(3Z)-N-[(1R)-1-(4-fluorophenyl)ethyl]-3-({4-[(furan-2-carbonyl)amino]-3,5-dimethyl-1H-pyrrol-2-yl}methylidene)-2-oxo-3,7-dihydro-2H-indole-5-carboxamide 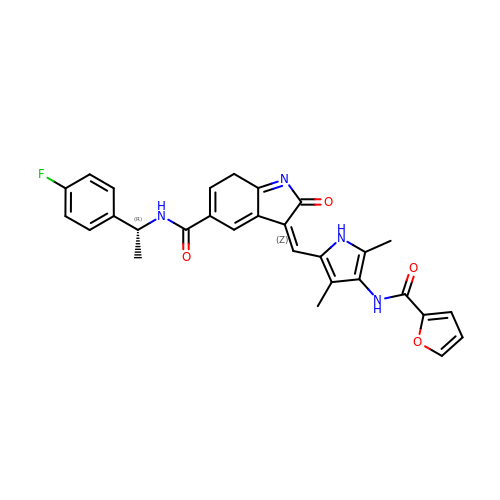| C29 H25 F N4 O4 | FLFIAOYKBCRNIL-LRSOKBAUSA-N> ADPGAPAPVNPCCYYPCQHQGICVRFGLDRYQCDCTRTGYSGPNCTIPEIWTWLRTTLRPSPSFIHFLLTHGRWLWDFVNATFIRDTLMRLVLTVRSNLIPSPPTYNIAHDYISWESFSNVSYYTRILPSVPRDCPTPMGTKGKKQLPDAEFLSRRFLLRRKFIPDPQGTNLMFAFFAQHFTHQFFKTSGKMGPGFTKALGHGVDLGH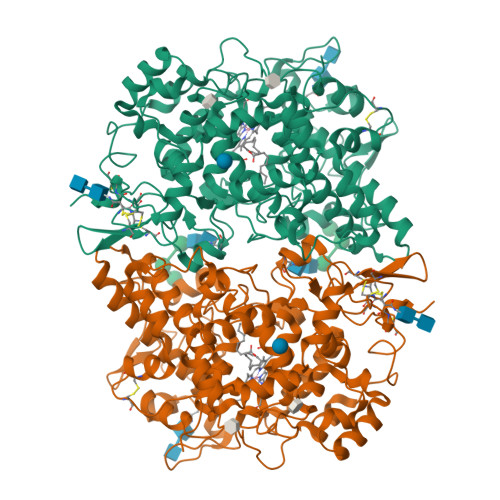IYGDNLERQYQLRLFKDGKLKYQMLNGEVYPPSVEEAPVLMHYPRGIPPQSQMAVGQEVFGLLPGLMLYATIWLREHNRVCDLLKAEHPTWGDEQLFQTARLILIGETIKIVIEEYVQQLSGYFLQLKFDPELLFGAQFQYRNRIAMEFNQLYHWHPLMPDSFRVGPQDYSYEQFLFNTSMLVDYGVEALVDAFSRQPAGRIGGGRNIDHHILHVAVDVIKESRVLRLQPFNEYRKRFGMKPYTSFQELTGEKEMAAELEELYGDIDALEFYPGLLLEKCHPNSIFGESMIEMGAPFSLKGLLGNPICSPEYWKASTFGGEVGFNLVKTATLKKLVCLNTKTCPYVSFHVPDPRQEDRPGVERPPTEL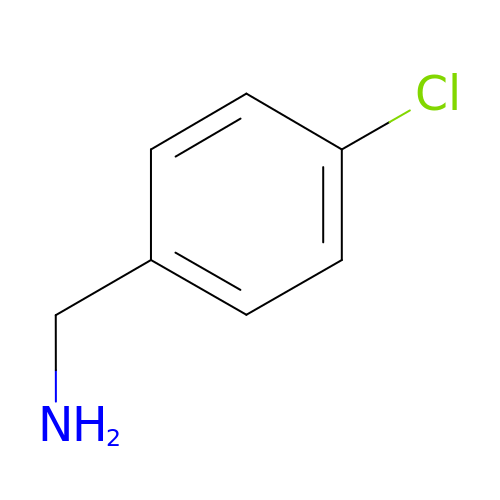1-(4-CHLOROPHENYL)METHANAMINE | C7 H8 Cl N | YMVFJGSXZNNUDW-UHFFFAOYSA-N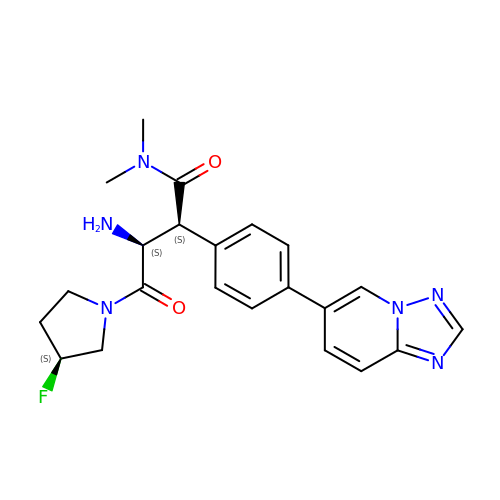6-(4-{(1S,2S)-2-AMINO-1-[(DIMETHYLAMINO)CARBONYL]-3-[(3S)-3-FLUOROPYRROLIDIN-1-YL]-3-OXOPROPYL}PHENYL)-1H-[1,2,4]TRIAZOLO[1,5-A]PYRIDIN-4-IUM | C22 H25 F N6 O2 | ZNHVIJAGMFQGMS-IHPCNDPISA-N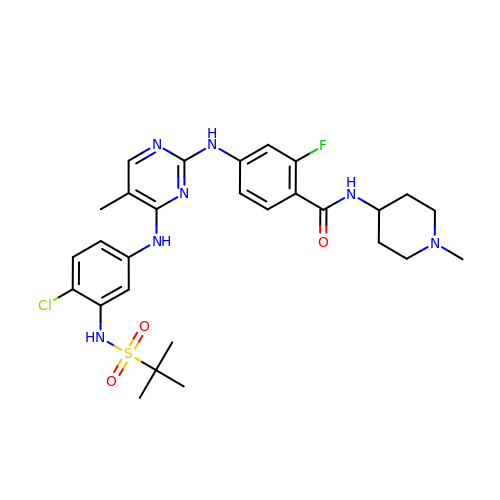4-[[4-[[3-(~{tert}-butylsulfonylamino)-4-chloranyl-phenyl]amino]-5-methyl-pyrimidin-2-yl]amino]-2-fluoranyl-~{N}-(1-methylpiperidin-4-yl)benzamide | C28 H35 Cl F N7 O3 S | RBZRCEPYYVFROZ-UHFFFAOYSA-N>MLQNIRIVLVETSHTGNMG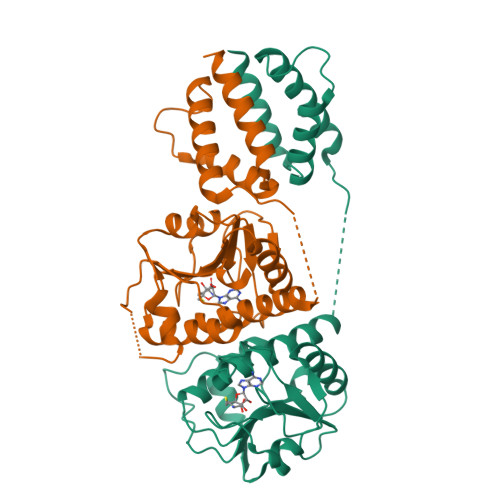SVARAMKTMGLTNLWLVNPLVKPDSQAIALAAGASDVIGNAHIVDTLDEALAGCSLVVGTSARSRTLPWPMLDPRECGLKSVAEAANTPVALVFGRERVGLTNEELQKCHYHVAIAANPEYSSLNLAMAVQVIAYEVRMAWLATQENGEQVEHEETPYPLVDDLERFYGHLEQTLLATGFIRENHPGQVMNKLRRLFTRARPESQELNILRGILASIEQQNKGNKAELEHHHHHH[2x]> MGKYNLILSEYLSFIYNSQSAVQIPIYYSSNSELENRCIEFHSKCLENSKNGLSLRKLFVEYNDVIENATLLSILSYSYDKYNAVERKLVKYAKGKPLEADLTVNELDYENNKMTSELFPTAEEYTDSLMDPAILTSLSSNLNAVMFWLEKHENDVAEKLKVYKRRLDLFTIVASTINKYGVPRHNAKYRYEYDVMKDKPYYLVTWANSSIEMLMSVFSHDDYLIAKELIVLSYSNRSTLAKLVSSPMSILVALVDINGTFITNEELELEFSNKYVRAIVPDQTFDELNQMLDNMRKAGLVDIPKMIQDWLVDRSIEKFPLMAKIYSWSFHVGFRKQKMLDAALDQLKTEYTENVDDEMYREYTMLIRDEVVKMLEEPVKHDDHLLRDSELAGLLSMSSASNGESRQLKFGRKTIFSTKKNMHVMDDMANERYTPGIIPPVNVDKPIPLGRRDVPGRRTRIIFILPYEYFIAQHAVVEKMLIYAKHTREYAEFYSQSNQLLSYGDVTRFLSNNTMVLYTDVSQWDSSQHNTQPFRKGIIMGLDILANMTNDAKVLQTLNLYKQTQINLMDSYVQIPDGNVIKKIQYGAVASG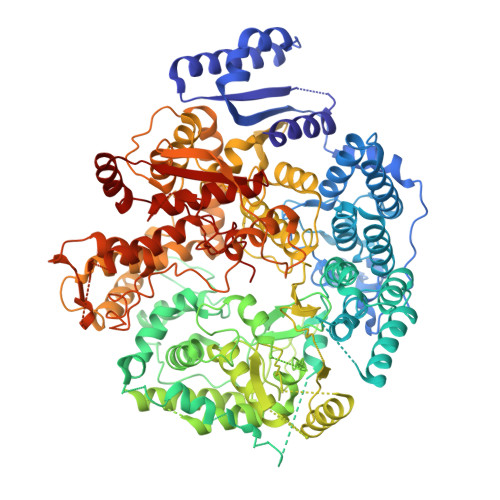EKQTKAANSIANLALIKTVLSRISNKHSFATKIIRVDGDDNYAVLQFNTEVTKQMIQDVSNDVRETYARMNAKVKALVSTVGIEIAKRYIAGGKIFFRAGINLLNNEKRGQSTQWDQAAILYSNYIVNRLRGFETDREFILTKIMQMTSVAITGSLRLFPSERVLTTNSTFKVFDSEDFIIEYGTTVDEVYIQRAFMSLSSQKSGIADEIAASSTFKNYVTRLSEQLLFSKNNIVSRGIALTEKAKLNSYAPISLEKRRAQISALLTMLQKPVTFKSSKITINDILRDIKPFFTVSDAHLPIQYQKFMPTLPDNVQYIIQCIGSRTYQIEDDGSKSAISRLISKYSVYKPSIEELYKVISLHENEIQLYLISLGIPKIDADTYVGSKIYSRDKYRILESYVYNLLSINYGCYQLFDFNSPDLEKLIRIPFKGKIPAVTFILHLYAKLEVINYAIKNGSWISLFCNYPKSEMIKLWKKMWNITSLRSPYTNANFFQEP>[2x]MKTLMVFDPAMAASTGVCGTDVDQALVDFSTDVQWLKQSGVQIERFNL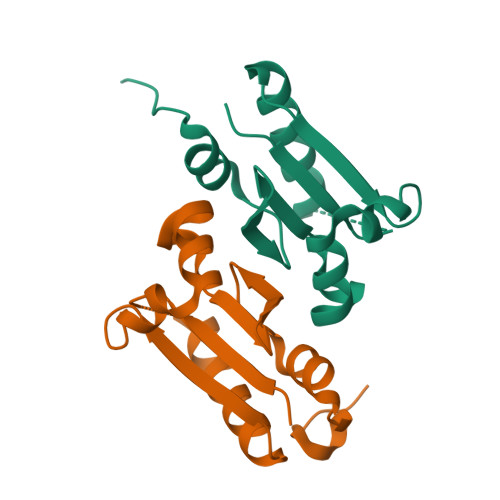AQQPMSFVQNEKVKAFIEASGAEGLPLLLLDGETVMAGRYPKRAELARWFGIPLDKVGLAPG>[2x]SGADDPNYFIGIKFRHIPYEYDVKIPHLTF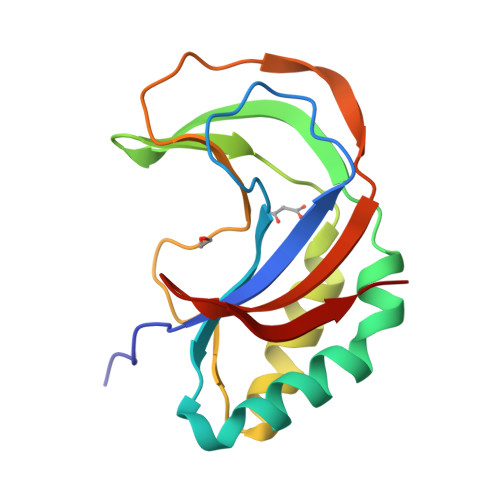GVLFISDNMIPDVVEIMKIMKKELFEMDITTSYTYMLSDGIYVANVSGVLATYFKMYNLFYKSQITFGQSRMFIPHITLSFSNNKTVRIESTRLKISSIYLRKIKGDTVFDMSE>[2x]RSWHYVEPKFL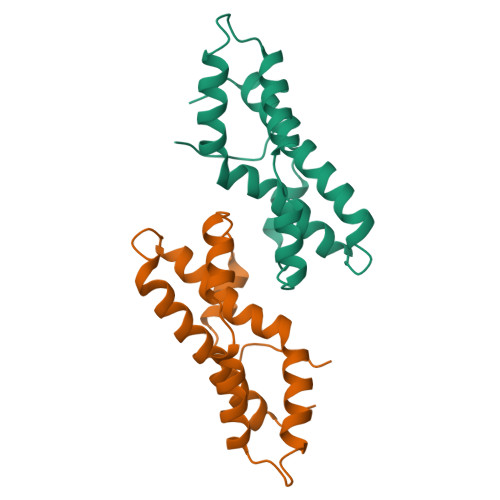NKAFEVALKVQIIAGFDRGLVKWLRVHGRTLSTVQKKALYFVNRRYMQTHWANYMLWINKKIDALGRTPVVGDYTRLGAEIGRRIDMAYFYDFLKDKNMIPKYLPYMEEINRMRPADVPVKYMGK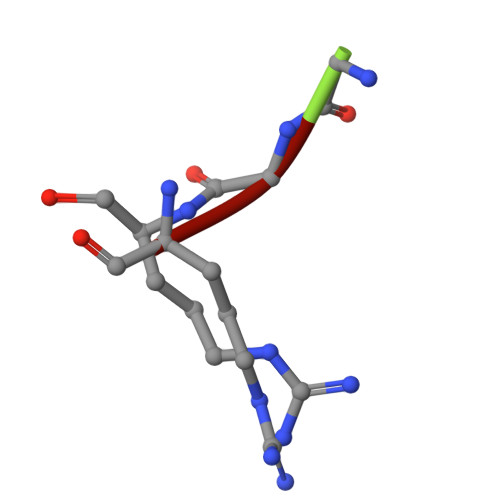> GGR N-(3-chloro-4-fluorophenyl)-3-[4-(dimethylamino)butanamido]-4-methoxybenzamide | C20 H23 Cl 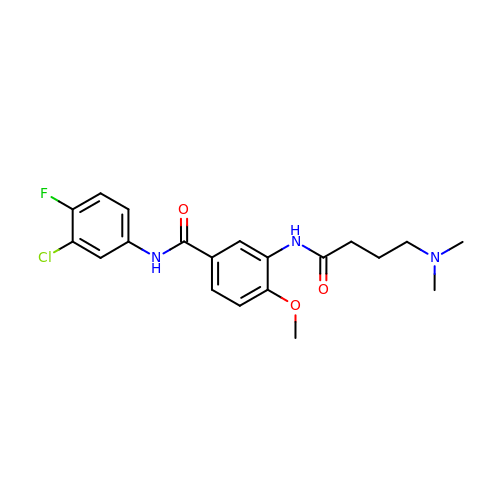F N3 O3 | VFCRGORDSAIMRG-UHFFFAOYSA-N> AVPAVGEDFPIDYADWLPKRDPNDRRRAGILLHPTSFPGPYGIGDLGPQAFKFLDWLHLAGCSLWQVLPLVPPGKRGNEDGSPYSGQDANCGNTLLISLEELVDDGLLKMEELPEPLPTDRVNYSTISEIKDPLITKAAKRLLSSEGELKDQLENFRRDPNISSWLEDAAYFAAIDNSVNTISWYDWPEPLKNRHLAALEEVYQSEKDFIDIFIAQQFLFQRQWKKVRDYARSKGISIMGDMPIYVGYHSADVWANKKQFLLNRKGFPLIVSGVPPDAFSETGQLWGSPLYDWKAMEKDGFSWWVRRIQRATDLFDEFRIDHFRGFAGFWAVPSEEK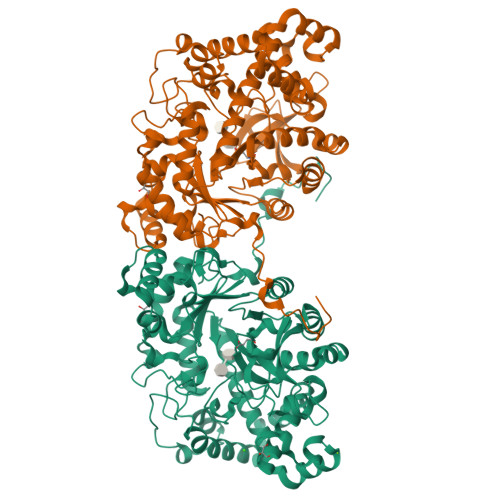IAILGRWKVGPGKPLFDAILQAVGKINIIAEDLGVITEDVVQLRKSIEAPGMAVLQFAFGSDAENPHLPHNHEQNQVVYTGTHDNDTIRGWWDTLPQEEKSNVLKYLSNIEEEEISRGLIEGAVSSVARIAIIPMQDVLGLGSDSRMNIPATQFGNWSWRIPSSTSFDNLDAEAKKLRDILATYGRL>MFPDLKGKRVLITGSSQGIGLATARL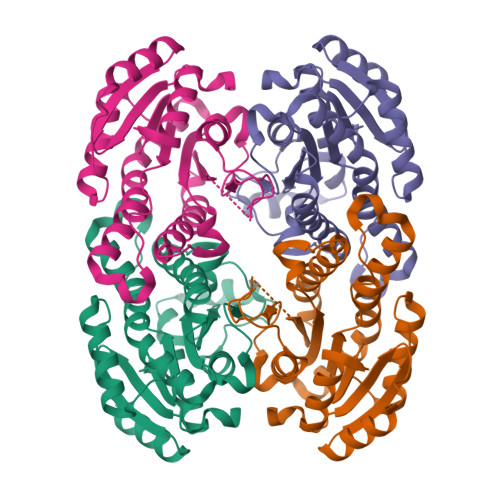FARAGAKVGLHGRKAPANIDETIASMRADGGDAAFFAADLATSEACQQLVDEFVAKFGGIDVLINNAGGLVGRKPLPEIDDTFYDAVMDANIRSVVMTTKFALPHLAAAAKASGQTSAVISTGSIAGHTGGGPGAGLYGAAKAFLHNVHKNWVDFHTKDGVRFNIVSPGTVDTAFHADKTQDVRDRISNGIPMGRFGTAEEMAPAFLFFASHLASGYITGQVLDINGGQYKH[2x]>GTDDATADSRKTYTLTDYLKNTYRLKLYSLRWISDHEYLYKQENNILVFNAEYGNSSVFLENSTFDEFGHSINDYSISPDGQFILLEYNYVKQWRHSYTASYDIYDLNKRQLITEERIPANTQWVTWSPVGHKLAYVWNNDIYVKIEPNLPSYRITWTGKEDIIYNGITDWVYEEEVFSAYSALWWSPNGTFLAYAQFNDTEVPLIEYSFYSDESLQYPKTVRVPYPKAGAVNPTVKFFVVNTDSLSSVTNATSIQITAPASMLIGDHYLCDVTWATQERISLQWLRRIQNYSVMDICDYDESSGRWNCLVARQHIEMSTTGWVGRFRPSEPHFTLDGNSFYKIISNEEGYRHICYFQIDKKDCTFITKGTWEVIGIEALTSDYLYYISNEYKGMPGGRNLYKIQLSDYTKVTCLSCELNPERCQYYSVSFSKEAKYYQLRCSGPGLPLYTLHSSVNDKGLRVLEDNSALDKMLQNVQMPSKKLDFIILAETKFWYQMILPPHFDKSKKYPLLLDVYAGPCSQKADTVFRLNWATYLASTENIIVASFDGRGSGYQGDKIMHAINRRLGTFEVEDQIEAARQFSKMGFVDNKRIAIWGWSYGGYVTSMVLGSGSGV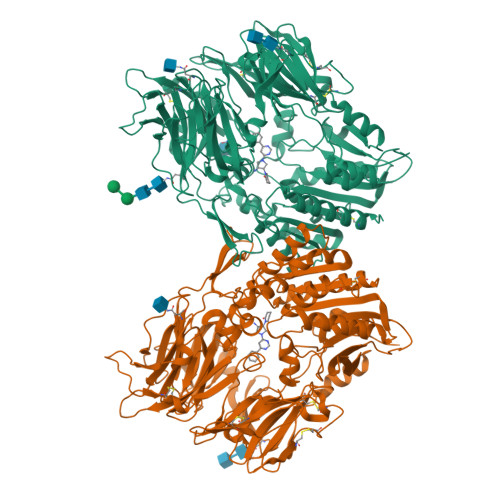FKCGIAVAPVSRWEYYDSVYTERYMGLPTPEDNLDHYRNSTVMSRAENFKQVEYLLIHGTADDNVHFQQSAQISKALVDVGVDFQAMWYTDEDHGIASSTAHQHIYTHMSHFIKQCFSLPLVPRGSHHHHHH[2x]IL‐6 is a cytokine exerting both immunostimulating and regenerating effects depending on the localization of the IL‐6 receptor. In vivo, IL‐6 is mainly targeted to the liver but can also be complexed by a soluble, circulating IL‐6 receptor. Although many of the biological effects of the human cytokine interleukin 6 (IL‐6) have been studied in detail, little is known about the influence of the glycans present on this glycoprotein. A library of glycoforms of human interleukin 6 (IL‐6) comprising complex and mannosidic N‐glycans was generated by semisynthesis.

We also attempted to crystallize a synthetic IL‐6 glycoform and started with IL‐61. The crystallization of an IL‐6 glycoform with a full‐length N‐glycan (data not shown) was not successful. The structure of IL‐61 (GlcNAc) did not resolve the flexible loop beyond Glu 50 (Ser 51‐Asn 59) but refinement to 2.0 Å showed low electron density for the GlcNAc residue indicating connectivity at the side chain amide. Notably, in both structures the unstructured loop region ends at Asn 60. In segment B the N‐terminal cysteine was protected by a mixed disulfide and the native methionine at position 48 was replaced with a norleucine, thus preventing undesired oxidation. The three segments were connected by sequential native chemical ligation followed by two‐step refolding. The glycoforms were characterized by LC‐MS, HR‐MS, SDS‐PAGE and CD‐spectroscopy indicating that the correct fold was attained and the formation of the disulfides was complete. The native helical fold of the set of IL‐6 glycoforms was independent of the glycan and only the overall intensity of the spectra varied to a small extent. The resulting hIL‐6 glycoproteins were of high‐purity and were properly folded according to CD‐spectroscopy, LC‐MS, HR‐MS and X‐ray crystallography (one structure). Despite the variations in the sugar part the activity of the individual glycoforms was nearly identical in the cellular assays indicating that the binding to the IL‐6 receptor and the formation of the signal‐transducing receptor complex should not be significantly affected by the various N‐glycan structures.

> VPPGEDSKDVAAPHRQPLTSSERIDKQIRYILDGISALRKETCNKSNLCESSKEALAENNLNLPKMAEKDGCFQSGFNEETCLVKIITGLLEFEVYLEYLQNRFESSEEQARAVQMSTKVLIQFLQKKAKNLDAITTPDPTTNASLLTKLQAQNQWLQDMTTHLILRSFKEFLQSSLRALRQM In humans, the CALHM family encompasses six paralogs, some of which function as non-selective channels that are permeable to large substances such as ATP. We identified the three paralogs, CALHM2, 4 and 6, to be highly expressed in this organ. The CALHM subunits thus constitute unique modular building blocks that assemble with different stoichiometries into large membrane channels. In contrast to previously described CALHM structures, where the oligomeric state of individual channels was described as uniform, our data show heterogeneous populations with CALHM4 and CALHM6 assembling as decameric and undecameric channels with similar abundance and CALHM2 as predominantly undecameric proteins with a smaller population of dodecamers (Figure 3—figure supplements 2–4 and 6). Despite the unknown activating stimuli, our study has provided insight into gating transitions of CALHM channels by showing two conformations with either a cylindrical pore of uniform large dimeter within the membrane that is constricted at the intracellular side as in case of CALHM4 and a conical pore that continuously narrows from its extracellular entry towards the cytoplasm as in case of CALHM6.

In each case, we found a heterogeneous, about equal distribution of particles with two distinct oligomeric states. The smaller particles are composed of decameric and the larger of undecameric assemblies, both of which we refer to as CALHM4 channels. In each structure, the subunits are arranged around a central axis of symmetry that defines the ion-conduction path. Both assemblies contain pairs of CALHM4 channels of the same size related by two-fold symmetry that interact via their cytoplasmic parts. In the plane of the membrane, the dimensions of decameric and undecameric CALHM4 channels amount to 110 Å and 120 Å respectively. The diameter at both entrances of the pore measures about 52 Å and 60 Å for decameric and undecameric assemblies respectively, thus defining the properties of an unusually large channel, which could be permeable to molecular substrates. Even at the constriction located at the intracellular membrane leaflet where the respective N-terminal helices NH project towards the pore axis, the decameric channels are about 20 Å and undecameric channels 30 Å wide. In our data, we find strong evidence for a layered distribution of density inside the pore within the presumed membrane region in non-symmetrized maps and after application of symmetry. This density is observed with similar properties in decameric and undecameric proteins in both datasets of CALHM4 obtained in either absence or presence of Ca2+. Collectively, our data are compatible with the presence of a lipid bilayer located within the pore region of CALHM4 channels, which could interfere with the diffusion of charged substances.

>[22x]MCPTLNNIVSSLQRNGIFINSLIAALTIGGQQLFSSSTFSCPCQVGKNFYYGSAFLVIPALILLVAGFALRSQMWTITGEYCCSCAPPYRRISPLECKLACLRFFSITGRAVIAPLTWLAVTLLTGTYYECAASEFASVDHYPMFDNVSASKREEILAGFPCCRSAPSDVILVRDEIALLHRYQSQMLGWILITLATIAALVSCCVAKCCSPLTSLQHCYWTSHLQNERELFEQAAEQHSRLLMMHRIKKLFGFIPGSEDVKHIRIPSCQDWKDISVPTLLCMGDDLQGHYSFLGNRVDEDNEEDRSRGIELKP>[2x]MARFEEQKLYIGGRYVEASSGATFETINPANGEVLAKVQRASREDVERAVQSAVEGQKVWAAMTAMQRSRILRRAVDILRERNDELAALETLDTGKPLAETRSVDIVTGADVLEYYAGLVPAIEGEQIPLRETSFVYTRREPLGVVAGIGAWNYPVQIALWKSAPALAAGNAMIFKPSEVTPLTALK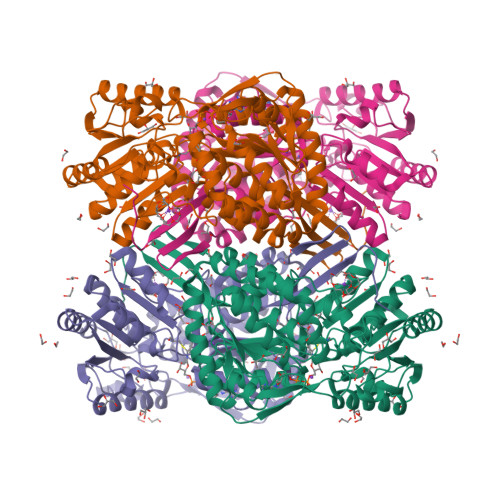LAEIYTEAGVPDGVFNVLTGSGREVGQWLTEHPLIEKISFTGGTSTGKKVMASASSSSLKEVTMELGGKSPLIIFPDADLDRAADIAVMANFFSSGQVCTNGTRVFIHRSQQARFEAKVLERVQRIRLGDPQDENTNFGPLVSFPHMESVLGYIESGKAQKARLLCGGERVTDGAFGKGAYVAPTVFTDCRDDMTIVREEIFGPVMSILVYDDEDEAIRRANDTEYGLAAGVVTQDLARAHRAIHRLEAGICWINTWGESPAEMPVGGYKQSGVGRENGLTTLAHYTRIKSVQVELGDYASVF>LGKFSQTCYNSAIQGSVLTSTCERTNGGYN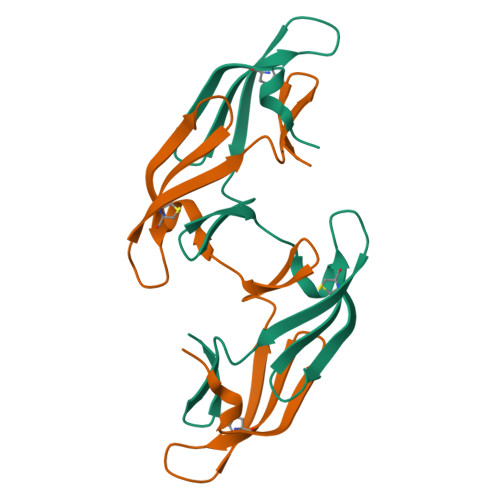TSSIDLNSVIENVDGSLKWQGSNFIETCRNTQLAGSSELAAECKTRAQQFVSTKINLDDHIANIDGTLKYE[4x]>[2x]GPEAEQQGRVFRYFGDKLLISEAKQSFTRVGENNLTCISCFQPVLNKYTFEESSNG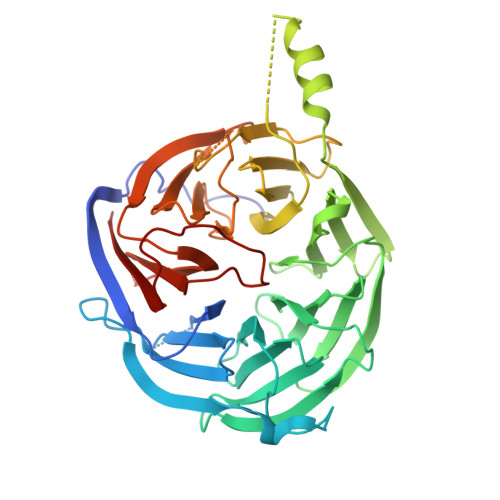DKNKGRLFAYTVSKDLQLTKYDITDFSKRPKKLKYAKGGAKYIPTSKHEYENTTEGHYDEILTVAASPDGKYVVTGGRDRKLIVWSTESLSPVKVIPTKDRRGEVLSLAFRKNSDQLYASCADFKIRTYSINQFSQLEILYGHHDIVEDISALAMERCVTVGARDRTAMLWKIPDETRLTFRGGDEPQKLLRRWMKENAKEGEDGEVKYPDESEAPLFFCEGSIDVVSMVDDFHFITGSDNGNICLWSLAKKKPIFTERIAHGILPEPSFNDISGETDEELRKRQLQGKKLLQPFWITSLYAIPYSNVFISGSWSGSLKVWKISDNLRSFELLGELSGAKGVVTKIQVVESGKHGKEKFRILASIAKEHRLGRWIANVSGARNGIYSAVIDQTGF>[2x]SNVPHKSSLPEGIRPGTVLAIRGLVPPNASRFHVNLLCGEEQGSDAALHFNPRLDTSEVVFNSKEQGSWGREERGPGVPFQRGQPFEV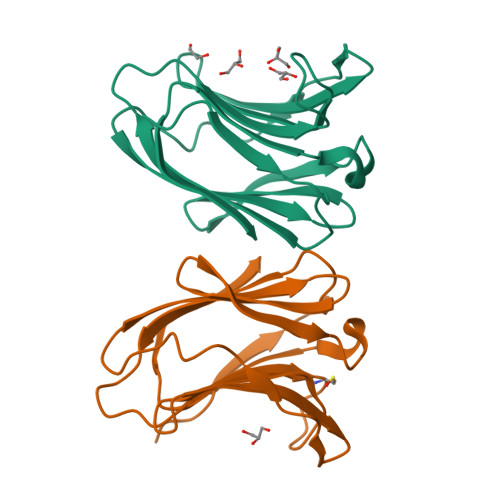LIIASDDGFKAVVGDAQYHHFRHRLPLARVRLVEVGGDVQLDSVRIF> MKKIEAIIRPFKLDEVKIALVNAGIVGMTVSEVRGFGRQKG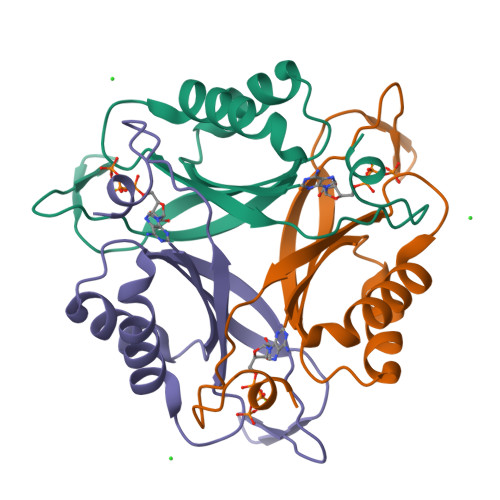QTERYRGSEYTVEFLQKLKLEIVVEDAQVDTVIDKIVAAARTGENGDGKIFVSPVDQTIRIRTGEKNADAIS> GNCKPPYSFSCLIFMAIEDSPTKRLPVKDIYNWILEHFPYFANAPTGWKNSVRHNLSLNKCFKKVDKERSQSIGKGSLWCIDPEYRQNLIQAL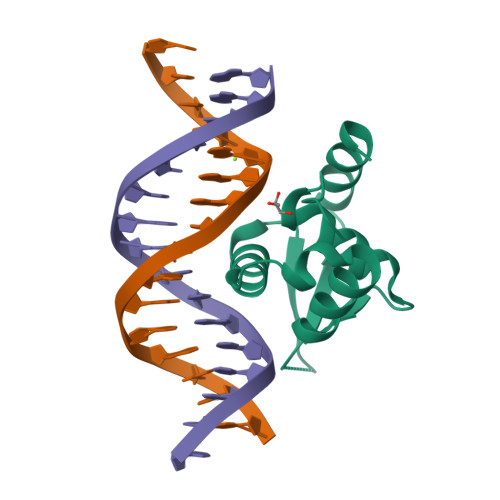KKTPYHP> QWYYIDGTRPQLGRN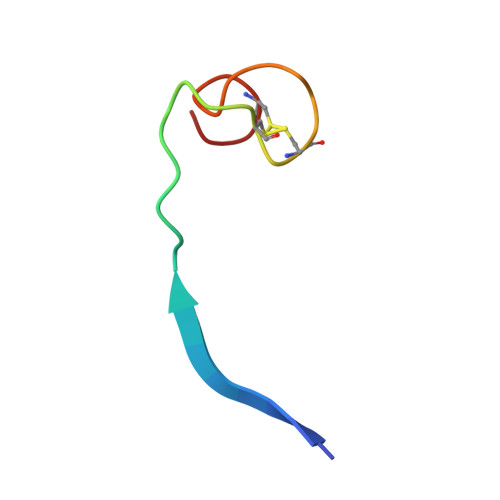DPCPCGSGKKFKKCCGQ>GSHMVLSNENLGQSLHQEGFSIPLLWLQNCLIRAADDREEDGCSQAVPLVPLTEENEEAMENEQFQQLLRKLGVRPP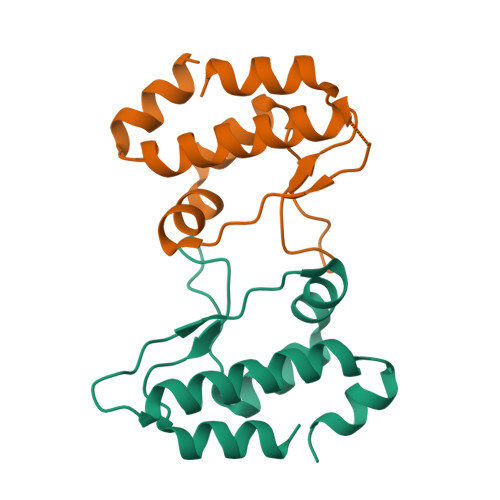ASGQETFWRIPAKLSPTQLRRAAASL[4x]> QDLALSCGTSEASADQDKKKWEPDTKFLKTGNSIHATATYQDPSLLSTVPYMTARIFTAPATYEIPIKGDKRHLLRLYFYPSTYTGLNISNSYFTVEANDVTLLSNFSAAITCQALTQAYLVKEYSLAPTDKDVLSIKFTPSDKYRDAFAFINGIEVIQMPELFDTAALVGFTDQTMDAKTANLQSMFRLNVGGQDIPGSQDSGGLTRTWYNDAPYIFSAGLGVTLQASNNFRINYQNMPVSIAPADIYKTARSQGPNGDINLKSNLTWMFQIDKNFTYILR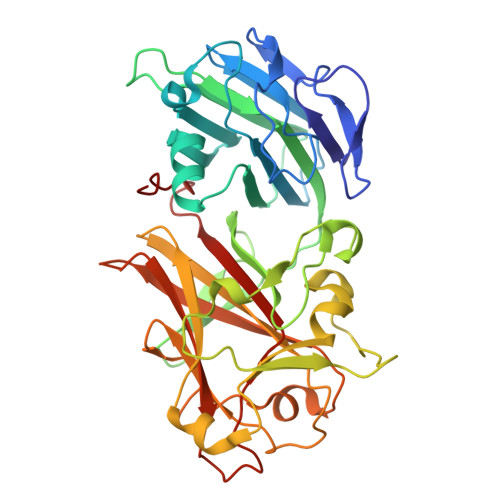LHFCEFQLSKINQKVFNIYINNRTAQADTTPADIIGWTGEKGIPMYKDYAIYVDANNGGEEITLQMTPSTFGQPEYYDSSLNGLEIFKMDTMKNLAGPNPEP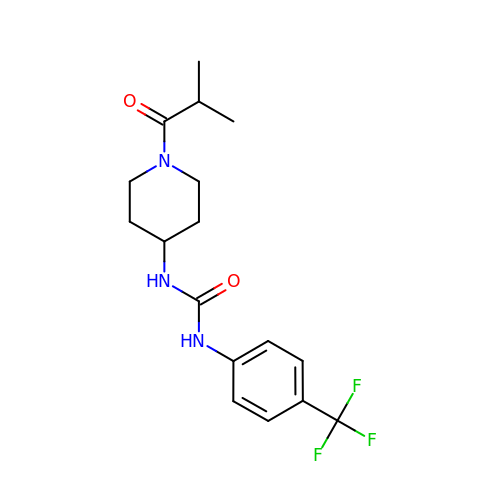1-[1-(2-methylpropanoyl)piperidin-4-yl]-3-[4-(trifluoromethyl)phenyl]urea | C17 H22 F3 N3 O2 | KKMHGEIPUCNGMV-UHFFFAOYSA-N>TAACCC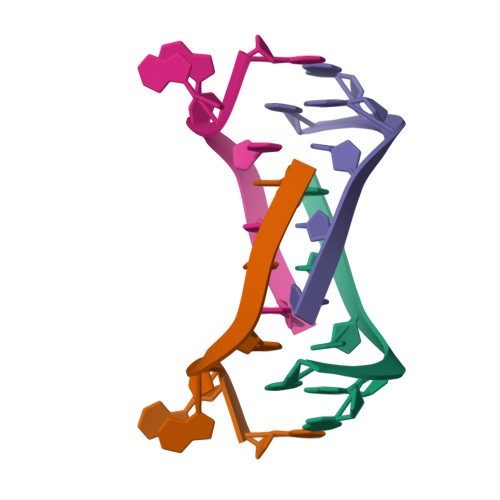[2x]>[2x]MGSHHHHHHGRSHHEEGHHDHEDLKDDHDPFLPEDHKKALFVYQKPALNNINFAFKMYRQLARDHPTENIVISPVSISSALALLSLGAKGHTHSQIVERLGYNTSEIPEQQIHESFHKQLDVVDDKDRDLEFEHGNALFTCKEHKIHQTFLDDAKKFYHSEVIPTDFKNTE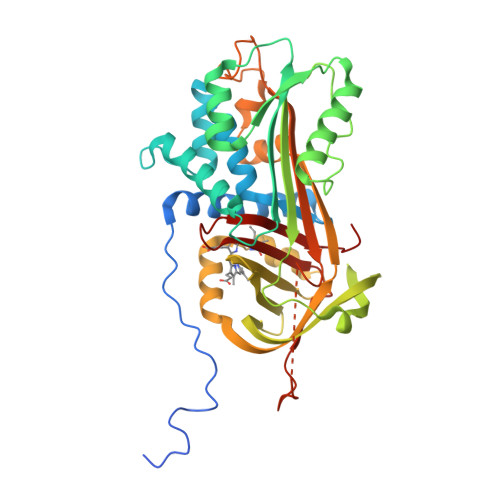EAKNQINSYVEKSTHGKITNILDSVDQDAMIALINFIYLRANWQHPFDEKLTKEGDFHVDKDTTVKVPFMRRRGIYKMAYTDDIIMVTIPYNGSVEMFLAMTKMGKLSELEQNLNRERSLKWREIMQYQLIDLSLPKLSVSGILNLKETLSKLGIVDVFSNHADLSGITDESHLKVSKAIHKAMMSFDEHGTEAAPATAAEADPLMLPPHFKFDYPFIFRVQDLKTKNPLLVGRIANPQK NALCN consists of a single polypeptide chain of 24 transmembrane helices (TM) that form four homologous functional repeats connected by intracellular linkers. NALCN is associated with several auxiliary subunits, including UNC80, UNC79, and FAM155A (Family with sequence similarity 155, member A). Together, they form a large protein complex termed the NALCN channelosome. In addition to its role in regulating neuronal excitability, NALCN is also important in many fundamental physiological processes, such as motor function, pain sensitivity and circadian rhythm.

Here, we report the cryo-EM structure of human NALCN in complex with FAM155A at an overall resolution of 3.1 Å. Three glycosylation sites (Asn210, Asn216, and Asn1064) were identified on NALCN and one glycosylation site (Asn217) on FAM155A. FAM155A sits above the pore domain of repeat IV of NALCN and forms extensive interactions with the ECLI, ECLIII, and ECLIV of NALCN. When the four VSDs are superimposed relative to An1 and CTC, all R4 residues are above the occluding residues on S2, reminiscent of up or depolarized states. Moreover, the S4-5I linker unexpectedly forms a flexible loop instead of a juxtamembrane helix as seen in the other three repeats of NALCN and other Nav/Cav structures. Notably, the unique structure of S4-5I and S5I results in a cavity that accommodates a lipid, which may contribute to the regulation of NALCN. We have assigned a total of ten lipid molecules in the structure. The key residues in the SF of NALCN responsible for the ion selectivity are E280/E554/K1115/E1389 (EEKE), distinct from DEKA in Nav channels and EEEE/EEDD in Cav channels. Surprisingly, although NALCN is supposed to conduct a “leak” current, the intracellular gate is closed, even more tightly than the closed Cav1.1. Notably, the lower gate is fully blocked by the III-IV linker.

> MLKRKQSSRVEAQPVTDFGPDESLSDNADILWINKPWVHSLLRICAIISVISVCMNTPMTFEHYPPLQYVTFTLDTLLMFLYTAEMIAKMHIRGIVKGDSSYVKDRWCVFDGFMVFCLWVSLVLQVFEIADIVDQMSPWGMLRIPRPLIMIRAFRIYFRFELPRTRITNILKRSGEQIWSVSIFLLFFLLLYGILGVQMFGTFTYHCVVNDTKPGNVTWNSLAIPDTHCSPELEEGYQCPPGFKCMDLEDLGLSRQELGYSGFNEIGTSIFTVYEAASQEGWVFLMYRAIDSFPRWRSYFYFITLIFFLAWLVKNVFIAVIIETFAEIRVQFQQMWGSRSSTTSTATTQMFHEDAAGGWQLVAVDVNKPQGRAPACLQKMMRSSVFHMFILSMVTVDVIVAASNYYKGENFRRQYDEFYLAEVAFTVLFDLEALLKIWCLGFTGYISSSLHKFELLLVIGTTLHVYPDLYHSQFTYFQVLRVVRLIKISPALEDFVYKIFGPGKKLGSLVVFTASLLIVMSAISLQMFCFVEELDRFTTFPRAFMSMFQILTQEGWVDVMDQTLNAVGHMWAPVVAIYFILYHLFATLILLSLFVAVILDNLELDEDLKKLKQLKQSEANADTKEKLPLRLRIFEKFPNRPQMVKISKLPSDFTVPKIRESFMKQFIDRQQQDTCCLLRSLPTTSSSSCDHSKRSAIEDNKYIDQKLRKSVFSIRARNLLEKETAVTKILRACTRQRMLSGSFEGQPAKERSILSVQHHIRQERRSLRHGSNSQRISRGKSLETLTQDHSNTVRYRNAQREDSEIKMIQEKKEQAEMKRKVQEEELRENHPYFDKPLFIVGREHRFRNFCRVVVRARFNASKTDPVTGAVKNTKYHQLYDLLGLVTYLDWVMIIVTICSCISMMFESPFRRVMHAPTLQIAEYVFVIFMSIELNLKIMADGLFFTPTAVIRDFGGVMDIFIYLVSLIFLCWMPQNVPAESGAQLLMVLRCLRPLRIFKLVPQMRKVVRELFSGFKEIFLVSILLLTLMLVFASFGVQLFAGKLAKCNDPNIIRREDCNGIFRINVSVSKNLNLKLRPGEKKPGFWVPRVWANPRNFNFDNVGNAMLALFEVLSLKGWVEVRDVIIHRVGPIHGIYIHVFVFLGCMIGLTLFVGVVIANFNENKGTALLTVDQRRWEDLKSRLKIAQPLHLPPRPDNDGFRAKMYDITQHPFFKRTIALLVLAQSVLLSVKWDVEDPVTVPLATMSVVFTFIFVLEVTMKIIAMSPAGFWQSRRNRYDLLVTSLGVVWVVLHFALLNAYTYMMGACVIVFRFFSICGKHVTLKMLLLTVVVSMYKSFFIIVGMFLLLLCYAFAGVVLFGTVKYGENINRHANFSSAGKAITVLFRIVTGEDWNKIMHDCMVQPPFCTPDEFTYWATDCGNYAGALMYFCSFYVIIAYIMLNLLVAIIVENFSLFYSTEEDQLLSYNDLRHFQIIWNMVDDKREGVIPTFRVKFLLRLLRGRLEVDLDKDKLLFKHMCYEMERLHNGGDVTFHDVLSMLSYRSVDIRKSLQLEELLAREQLEYTIEEEVAKQTIRMWLKKCLKRIRAKQQQSCSIIHSLRESQQQELSRFLNPPSIETTQPSEDTNANSQDNSMQPETSSQQQLLSPTLSDRGGSRQDAADAGKPQRKFGQWRLPSAPKPISHSVSSVNLRFGGRTTMKSVVCKMNPMTDAASCGSEVKKWWTRQLTVESDESGDDLLDILEDEVDAGSDYKDDDDKGSDYKDDDDK;> MTRGAWMCRQYDDGLKIWLAAPRENEKPFIDSERAQKWRLSLASLLFFTVLLSDHLWFCAEAKLTRARDKEHQQQQRQQQQQQQQQRQRQQQQQQRRQQEPSWPALLASMGESSPAAQAHRLLSASSSPTLPPSPGDGGGGGGKGNRGKDDRGKALFLGNSAKPVWRLETCYPQGASSGQCFTVENADAVCARNWSRGAAGGDGQEVRSKHPTPLWNLSDFYLSFCNSYTLWELFSGLSSPNTLNCSLDVVLKEGGEMTTCRQCVEAYQDYDHHAQEKYEEFESVLHKYLQSEEYSVKSCPEDCKIVYKAWLCSQYFEVTQFNCRKTIPCKQYCLEVQTRCPFILPDNDEVIYGGLSSFICTGLYETFLTNDEPECCDVRREEKSNNPSKGTVEKSGSCHRTSLTVSSATRLCNSRLKLCVLVLILLHTVLTASAAQNTAGLSFGGINTLEENSTNEELEDEVDAGSDYKDDDDKGSDYKDDDDK> GSHMIYSEFIMDYSKLKKFHGKIENAHKVEEGKNLSCGDEVTLYFLFDGDKIVDVKFEGHGCAISQA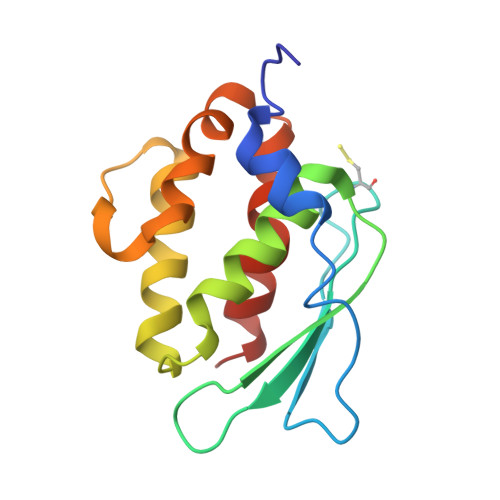STNVMIEQIIGKTKQEALEMMKNAENMMLGKEFDENVLGPIINFYDVKNYPMRVKCFLLPWKTLEIALKNE In this work, we exhaustively probe the ability of all 36 immobile HJ sequences to form DNA crystals in two different designed systems. Three separate self-assembling DNA crystal systems are described in this report: the “4 × 5” and “4 × 6” designs (collectively referred to as the 4 × N systems), and a third construct with a “scrambled” sequence variant of the 4 × 6 lattices. Self-assembly was mediated by three constituent oligonucleotides: (S1) containing four sequence repeats of either 5 or 6 bases; (S2) composed of 21 bases containing complementary regions to both (S1); and (S3) which forms the second junction crossover. The HJ serves as the fundamental component at the core of each unit, and the ultimate assembly of the full lattice is facilitated by the complementary 2-base sticky ends that tail each duplex.

Each asymmetric unit could be defined as either a HJ containing 10 and 11 bp on each arm, or as a 21-bp linear duplex. The 4 × 5 system robustly crystallized with 75% of the junctions, and we obtained crystals in all but 9 of 36 sequences. Of the resulting structures, 18 exhibited P32 symmetry with average cell dimensions a = b = 68.85 Å c = 60.09 Å, with only nine retaining the original P3221 symmetry with average cell edges a = b = 68.17 Å c = 60.60 Å. Although the cell parameters between the two symmetries were virtually indistinguishable, the differences between the periodicity of the lattices is dramatic, with vastly different cavity sizes.

> GAGCAGACTTGACAGCACTCA;> TGTCA;> TCTGAGTGC;> AGTCTGC> MVPISPIETVPVKLKPGMDGPKVKQWPLTEEKIKALVEICTEMEKEGKISKIGPENPYNTPVFAIKKKWRKLVDFRELNKRTQDFWEVQLGIPHPAGLKKKKSVTVLDVGDAYFSVPLDEDFRKYTAFTIPSINNETPGIRYQYNVLPQGWKGSPAIFQSSMTKILEPFAAQNPDIVIYQYMDDLYVGSDLEIGQHRTKIEELRQHLLRWGLTTPAKEPPFLWMGYELHPDKWTVQPIVLPEKDSWTVNDIQKLVGKLNWASQIYPGIKVRQLSKLLRKALTEVIPLTEEAELELAENREILKEPVHGVYYDPSKDLIAEIQKQGQGQWTYQIYQEPFKNLKTGKYARMRGAHTNDVKQLTEAVQKITTESIVIWGKTPKFKLPIQKETWETWWTEYWQATWIPEWEFVNTPPLVKLWYQLEKEPIVGAETFYVDGAANRETKLGKAGYVTNKGRQKVVPLTNTTNQKTELQAIYLALQDSGLEVNIVTDSQYALGIIQAQPDKSESELVNQIIEQLIKKEKVYLAWVPAHKGIGGN;> IETVPVKLKPGMDGPKVKQWPLTEEKIKALVEICTEMEKEGKISKIGPENPYNTPVFAIKKKDSTKWRKLVDFRELNKRTQDFWEVQLGIPHPAGLKKKKSVTVLDVGDAYFSVPLDEDFRKYTAFTIPSINNETPGIRYQYNVLPQGWKGSPAIFQSSMTKILEPFKKQNPDIVIYQYMDDLYVGSDLEIGQHRTKIEELRQHLLRWGLFLWMGYELHPDKWTVQPIVLPEKDSWTVNDIQKLVGKLNWASQIYPGIKVRQLSKLLRGTKALTEVIPLTEEAELELAENREILKEPVHGVYYDPSKDLIAEIQKQGQGQWTYQIYQEPFKNLKTGKYARMRGAHTNDVKQLTEAVQKITTESIVIWGKTPKF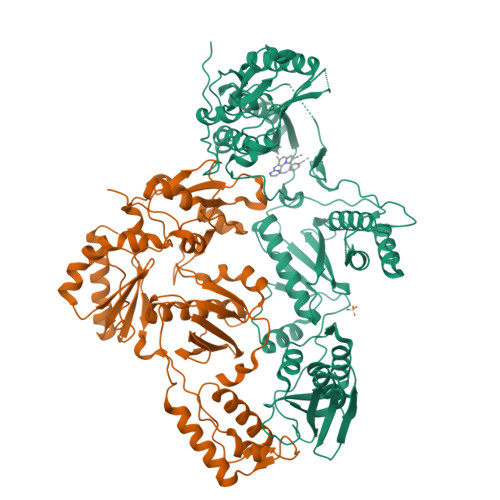KLPIQKETWETWWTEYWQATWIPEWEFVNTPPLVKLWYQ> GAMEKFKTLLYDIPIECMEVSEEIISYAKLQLGKKLNDSIYVSLTDHINFAIQRNQKGLDIKNALLWET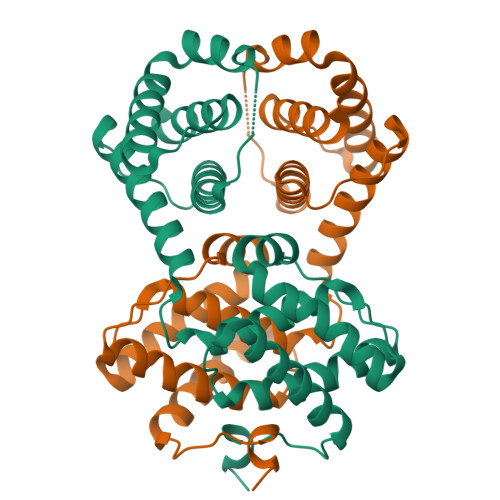KRLYKDEFAIGKEALVMVKNKTGVSLPEDEAGFIALHIVNAELNEEMPNIINITKVMEEILSIVKYHFKIEFNEESLHYYRFVTDLKFFAQRLFNGTHMESEDDFLLDTVKEKYHRAYECTKKIQTYIEREYEHKLTSDELLYLTIDIERVVKQA> GLRERCVRNYGHEFCQNW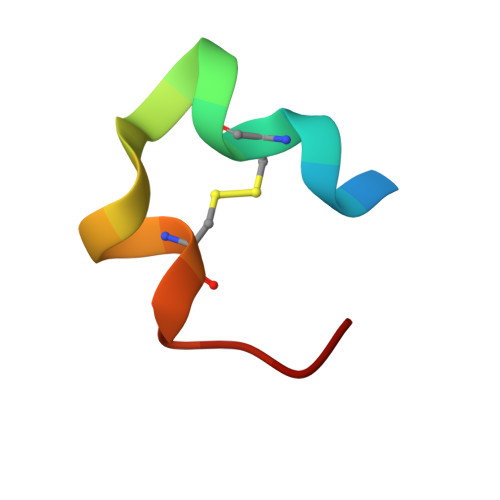YW> SLQPLPPTAFTPNGTYLQHLARDPTSGTLYLGATNFLFQLSPGLQLEATVSTGPVL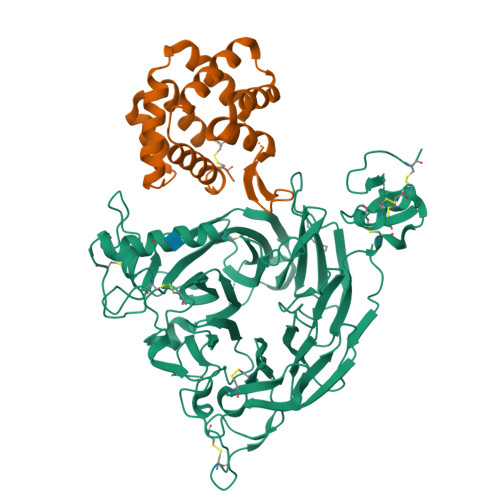DSRDCLPPVMPDECPQAQPTNNPNQLLLVSPGALVVCGSVHQGVCEQRRLGQLEQLLLRPERPGDTQYVAANDPAVSTVGLVAQGLAGEPLLFVGRGYTSRGVGGGIPPITTRALWPPDPQAAFSYEETAKLAVGRLSEYSHHFVSAFARGASAYFLFLRRDLQAQSRAFRAYVSRVCLRDQHYYSYVELPLACEGGRYGLIQAAAVATSREVAHGEVLFAAFSSAAPPTVGRPPSAAAGASGASALCAFPLDEVDRLANRTRDACYTREGRAEDGTEVAYIEYDVNSDCAQLPVDTLDAYPCGSDHTPSPMASRVPLEATPILEWPGIQLTAVAVTMEDGHTIAFLGDSQGQLHRVYLGPGSDGHPYSTQSIQQGSAVSRDLTFDGTFEHLYVMTQSTLLKVPVASCAQHLDCASCLAHRDPYCGWCVLLGRCSRRSECSRGQGPEQWLWSFQPELGCLQTRENLYFQ;> SEICPSFQRVIETLLMDTPSSYEAAMELFSPDQDMREAGAQLKKLVDTLPQKPRESIIKLMEKIAQSSLSGWRPYIERWTGRLIVGSPSFQRVIETLLMDTPSSYEAAMELFSPDQDMREAGAQLKKLVDTLPQKPRESIIKLMEKIAQSSLCNHHHHHH> MKKQNDIPQPIRGDKGATVKIPRNIERDRQNPDMLVPPETDHGTVSNMKFSFSDTHNRLEKGGYAREVTVRELPISENLASVNMRLKPGAIRELHYHKEAEWAYMIYGSARVTIVDEKGRSFIDDVGEGDLWYFPSGLPHSIQALEEGAEFLLVFDDGSFSENSTFQLTDWLAHTPKEVIAANFGVTKEEISNLPGKEKYIFENQLPGSLKDDIVEGPNGEVPYPFTYRLLEQEPIESEGGKVYIADSTNFKVSKTIASALVTVEPGAMRELHWHPNTHEWQYYISGKARMTVFASDGHARTFNYQAGDVGYVPFAMGHYVENIGDEPLVFLEIFKDDHYADVSLNQWLAMLPETFVQAHLDLGKDFTDVLSKEKHPVVKKKCSK

The hexameric low-pH stress response enzyme oxalate decarboxylase catalyzes the decarboxylation of the oxalate mono-anion in the soil bacterium Bacillus subtilis. A single protein subunit contains two Mn-binding cupin domains, and catalysis depends on Mn(III) at the N-terminal site. A π-stacked tryptophan pair (W96/W274) links two neighboring protein subunits together, thus reducing the Mn-to-Mn distance from 25.9 Å (intrasubunit) to 21.5 Å (intersubunit). The present study suggests a mechanistic function for the C-terminal Mn as an electron hole donor for the N-terminal Mn.

Site-directed replacement of tryptophan by phenylalanine was used to inactivate LRET while replacement with tyrosine was used as a potential positive control owing to its similar reduction potential compared with tryptophan. Since tyrosine has a redox potential similar to that of tryptophan it was expected to rescue activity. Of interest, the single W→Y mutants (W96Y and W274Y) have predicted hopping rates approximately the same as in the WT simulations, confirming our premise that replacing tryptophan with tyrosine will have little effect on the overall electron hopping rates, assuming that a proton acceptor is available to establish a neutral tyrosyl radical as the hopping intermediate. As expected, the W→Y single mutations rescue catalytic efficiency to almost WT levels. X-ray crystallography was carried out on single crystals of the W96F and W96Y forms to determine the structure of the W mutant proteins. W96F and W96Y mutants share the wildtype tertiary structure. Significantly, the π-stacking of W274 with the substituted phenylalanine (W96F) and tyrosine (W96Y) aromatic ring system was conserved. The average distance of the aromatic planes within each dimer differed only marginally by ∼ 0.1 Å or less. X-ray crystallography was used to confirm that the quaternary structure was not significantly disturbed by the mutations.>GFKQDIATLRGDLRTYAQDIFLAFLNKYPDEKRNFKNFVGKSDQELKSMAKFGDHTEKVFNLMMEVADRATDCVPLASDASTLVQMKQH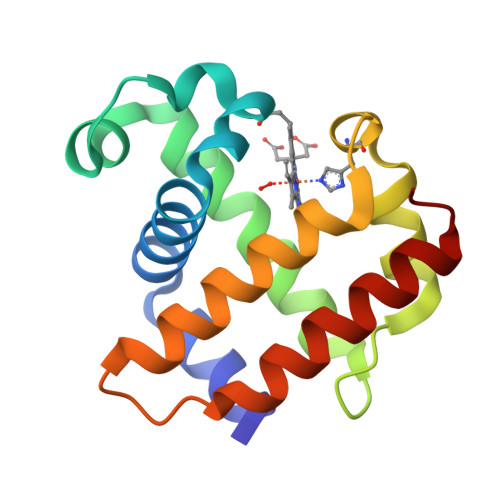SGLTTGNFEKLFVALVEYMRASGQSFDSQSWDRFGKNLVSALSSAGMK[2x]> GAQVSTQKSGSHENQNILTNGSNQTYTVINYYKDAASSSSAGQSFSMDPSKFTEPVKDLML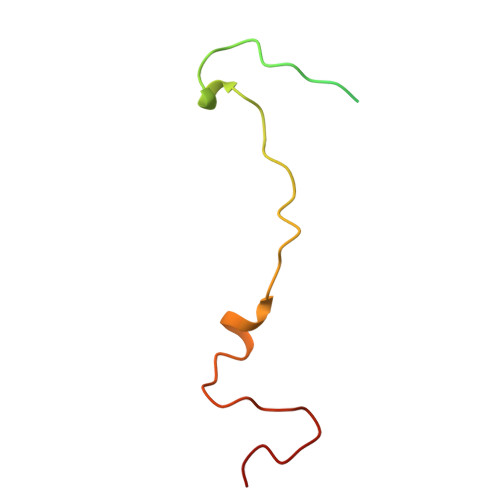KGAPALN>[2x]APTAKLANGDTITGLNAIINEAFLGIPFAEPPVGNLRFKDPVPYSGSLNGQKFTSYGPSCMQQNPEGTFEENLGKTALDLVMQSKVFQAVLPQSEDCLTINVVRPPGTKAGANLPVMLWIFGGGFEIGSPTIFPPAQMVTKSVLMGKPIIHVAVNYRV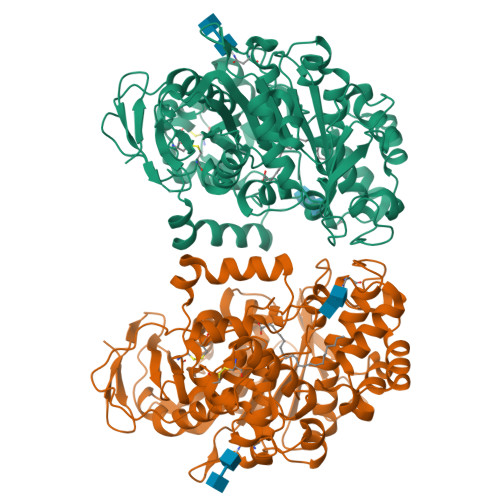ASWGFLAGDDIKAEGSGNAGLKDQRLGMQWVADNIAGFGGDPSKVTIFGESAGSMSVLCHLIWNDGDNTYKGKPLFRAGIMQSGAMVPSDPVDGTYGNEIYDLFVSSAGCGSASDKLACLRSASSDTLLDATNNTPGFLAYSSLRLSYLPRPDGKNITDDMYKLVRDGKYASVPVIIGDQNDEGTIFGLSSLNVTTNAQARAYFKQSFIHASDAEIDTLMAAYPQDITQGSPFDTGIFNAITPQFKRISAVLGDLAFIHARRYFLNHFQGGTKYSFLSKQLSGLPIMGTFHANDIVWQDYLLGSGSVIYNNAFIAFATDLDPNTAGLLVNWPKYTSSSQSGNNLMMINALGLYTGKDNFRTAGYDALMTNPSSFFV> G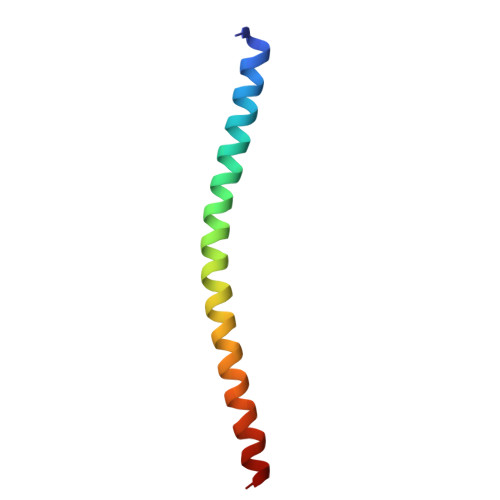SEFKENIINDLSDKLKSTMQQQERDKDLIESLSEDRARLLEEKKKLEEEVSKLRSS> PKHEFSVDMTCGGCAEAVSRVLNKLGGVKYDIDLPNKKVCIESEHSMDTLLATLKKTGKTVSYLGLEI;> VNSVTISVEGMTCNSCVWTIEQQIGKVNGVHHIKVSLEEKNATIIYDPKLQTPKTLQEAID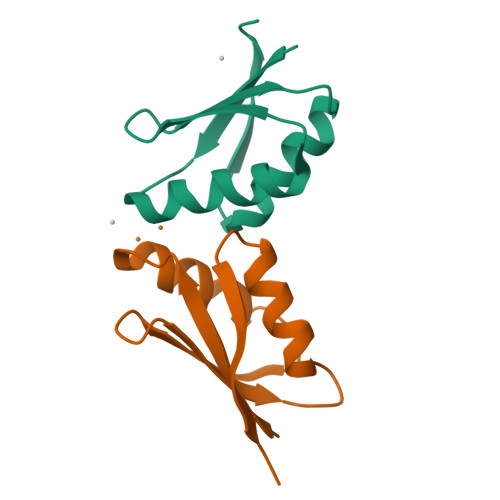DMGFDAVIHNIEGR>[3x]MGSSDS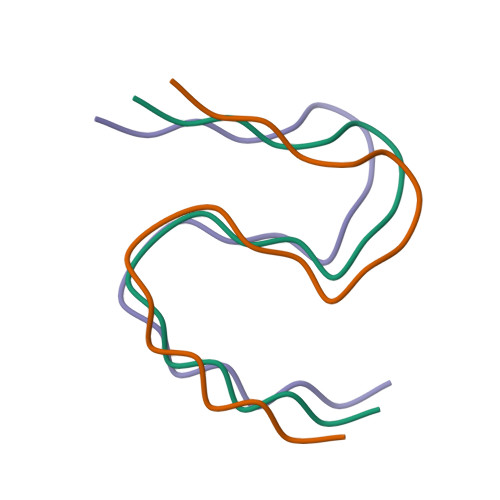MAQPPQTPETSTFRNQMPSPTSTGTPSPGPRGNQGAERQGMNWSCRTPEPNPVTGRPLVNIYNCSGVQVGDNNYLTMQQTTALPTWGLAPSGKGRGLQHPPPVGSQEGPKDPEAWSRPQGWYNHSGKLEHHHHHH>[2x]MATHKPINILEAFAAAPPPLDYVLPNMVAGTVGALVSPGGAGKSMLALQLAAQIAGGPDLLEVGELPTGPVIYLPAEDPPTAIHHRLHALGAHL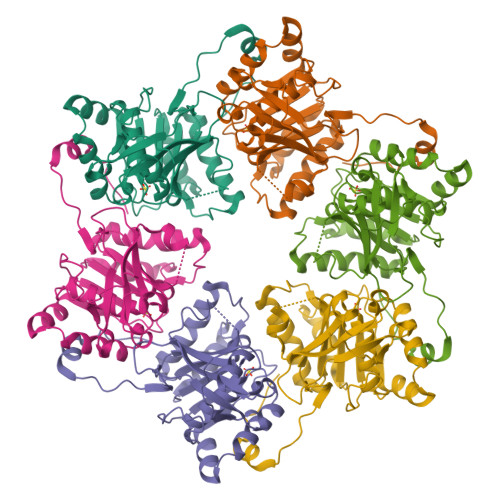SAEERQAVADGLLIQPLIGSLPNIMAPEWFDGLKRAAEGRRLMVLDTLRRFHIEEENASGPMAQVIGRMEAIAADTGCSIVFLHHASKGAAMMGAGDQQQASRGSSVLVDNIRWQSYLSSMTSAEAEEWGVDDDQRRFFVRFGVSKANYGAPFADRWFRRHDGGVLKPAVLERQRKSKGVPRGEA> APA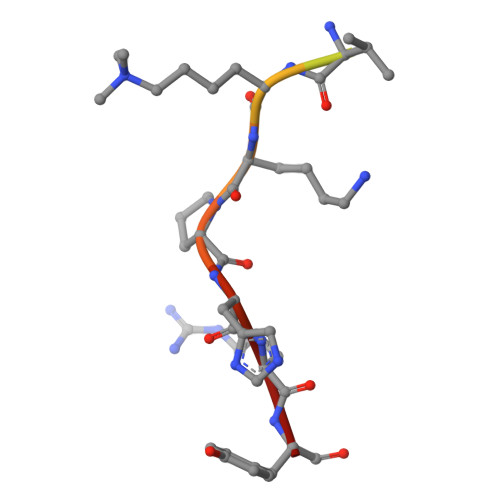TGGVKKPHRY>[2x]MPLLDSFAVDHTRMQAPAVRTAKTMNTPHGDAITVFDLRFCIPNKEVMPEKGIHTLEHLFAGFMRDHLNGNGVEIIDISPMGCRTGFYMSLIGTPDEQRVADAWKAAMADVLKVQDQNQI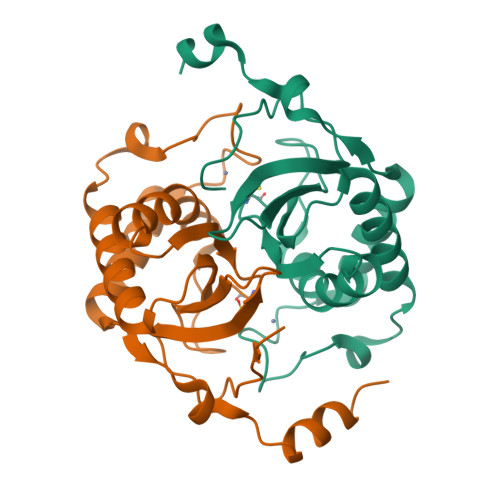PELNVYQCGTYQMHSLSEAQDIARHILERDVRVNSNKELALPKEKLQELHILEHHHHHH> KETAAAKFERQH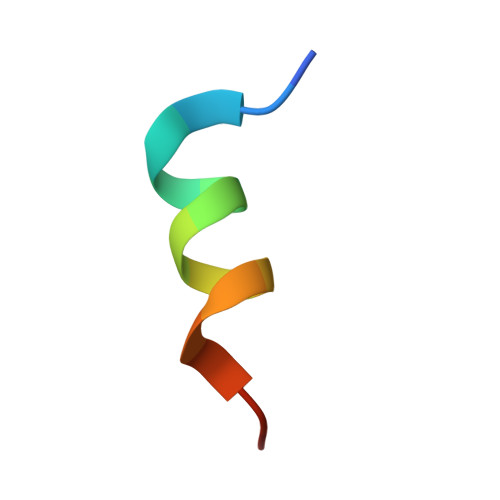FDSX Structurally, HDAC6 is a zinc-dependent metallohydrolase with an atypical complex domain organization that interacts predominantly with cytosolic substrates, including tubulin, cortactin, and peroxiredoxins. The catalytic activity of HDAC6 toward acetylated substrates has been studied both experimentally and computationally. Zinc-dependent histone deacetylases (HDACs) play critical roles in numerous (patho)physiological processes through the deacylation of lysine residues of their substrate proteins. Herein, we report on the synthesis and biochemical, crystallographic, and computational characterization of a series of oxadiazole-based inhibitors selectively targeting the HDAC6 isoform. Surprisingly, but in line with a very recent finding reported in the literature, a crystal structure of the HDAC6/inhibitor complex revealed that hydrolysis of the oxadiazole ring transforms the parent oxadiazole into an acylhydrazide through a sequence of two hydrolytic steps.

To elucidate the binding mode of inhibitor 8 in the HDAC6 active site, we co-crystallized 8 with the catalytic DD2 domain of the wild-type zebrafish orthologue (zHDAC6; amino acids 440–798). The crystal structure of the zHDAC6/inhibitor complex was solved by molecular replacement to the resolution limit of 1.35 Å. Surprisingly, the Fo–Fc electron density peaks in the vicinity of the active-site zinc ion revealed that the oxadiazole ring of the parent compound 8 had been hydrolyzed into a hydrazide reaction product (4, identified later). Once we had confirmed the chemical nature of the product by liquid chromatography–mass spectrometry (LC–MS)/MS, it was modeled into well-resolved Fo–Fc positive electron density peaks in the later stages of the refinement. The hydrazide group of 4 coordinates the active-site Zn2+ ion in a bidentate fashion, with an interatomic distance of 2.6 and 2.1 Å between the Zn2+ ion and the C=O and the terminal NH2 group of the hydrazide, respectively. Furthermore, the C=O group accepts a hydrogen bond from the hydroxyl group of Y745 (2.6 Å), and the N–N group forms hydrogen bonds with the imidazole ring present in the side chains of H573 (2.9 Å) and H574 (2.7 Å). The chlorophenyl moiety of the cap group of the inhibitor is positioned within van der Waals distances from the side chains of H463, F583, P464, and L712 (modeled in two conformations) of the L1-loop pocket. One of the more notable features here is the T-shaped π–π stacking interaction between the chlorophenyl group and the side chain of F583 at a distance of 5.1 Å between the aromatic ring centers. At the same time, the methylsulfonyl group is solvent exposed and does not contribute to interactions with the enzyme. The pyridine ring present in the linker engages in parallel π–π stacking with side chains of F583 and F643 lining the entrance tunnel, with distances of 4.0 and 4.2 Å between the respective aromatic residues.

> SSPITGLVYDQRMMLHHNMWDSHHPELPQRISRIFSRHEELRLLSRCHRIPARLATEEELALCHSSKHISIIKSSEHMKPRDLNRLGDEYNSIFISNESYTCALLAAGSCFNSAQAILTGQVRNAVAIVRPPGHHAEKDTACGFCFFNTAALTARYAQSITRESLRVLIVDWDVHHGNGTQHIFEEDDSVLYISLHRYEDGAFFPNSEDANYDKVGLGKGRGYNVNIPWNGGKMGDPEYMAAFHHLVMPIAREFAPELVLVSAGFDAARGDPLGGFQVTPEGYAHLTHQLMSLAAGRVLIILEGGYNLTSISESMSMCTSMLLGDSPPSLDHLTPLKTSATVSINNVLRAHAPFWSSLR> RSATPQCKEEEYPVGTECCPKCSPGYRVKQACGELTGTVCVPCAPRTFSAHLNGLSKCLPCRPCDPAMGLVIRRDCSSTENTECGCDQGHFCVSEKGDDCVECQPH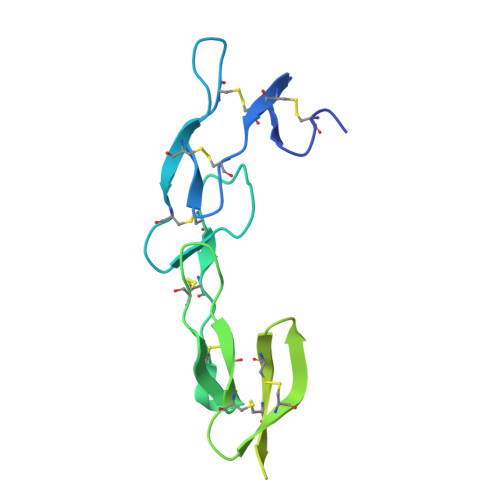TTCRPGQRVQERGTERQDTVCEDCQPGTFSPNGTLGECRPWTKCSGLFEMEVEPGTSSTDVTCSSSRENLYFQSNTGHHHHHH> VEWSTAERSAIAGLWGKISVDEIGPQALSRLLIVYPWTQRHFAAFG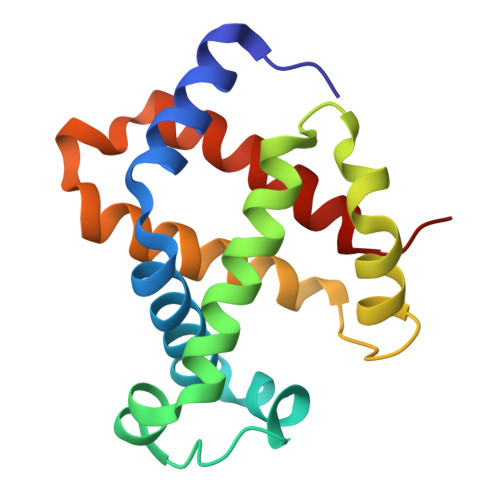NLSSPAAINGNPKVAHHGKVVMGGLERAIKNMDNIKAAYSSLSVMHSEKLHVDPDNFRLLADCITVCVAMKFGPSAFTPDVQEAWQKFLAVVVAALSRYH> SCDLNATNYIRGCQSKTYDGKIFPGKGGEKQWICKDTIIHGDTNGACIPPRTQNLCVGELWDKSYGGRSNIKNDTKELLKEKIKNAIHKETELLYEYHDTGTAIISKNDKKGQKGKNDPNGLPKGFCHAVQRSFIDYKNMILGTSVNIYEHIGKLQEDIKKIIEKGTPQQKDKIGGVGSSTENVNAWWKGIEREMWDAVRCAITKINKKNNNSIFNGDECGVSPPTGNDEDQSVSWFKEWGEQFCIERLRYEQNIREACTIN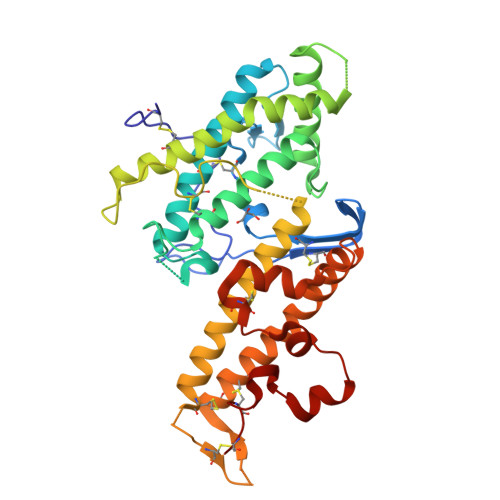GKNEKKCINSKSGQGDKIQGACKRKCEKYKKYISEKKQEWDKQKTKYENKYVGKSASDLLKENYPECISANFDFIFNDNIEYKTYYPYGDYSSICSCE>[2x]MLLEAIFHEAK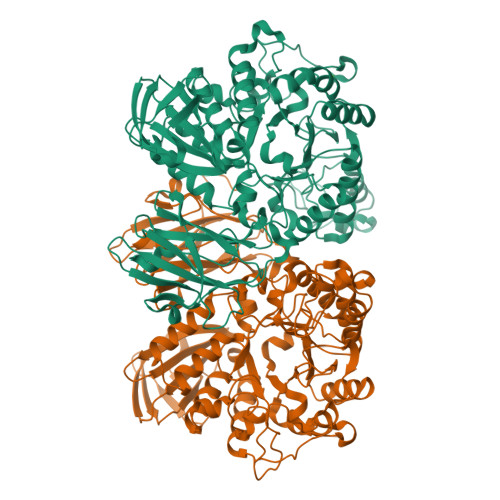GSYAYPISETQLRVRLRAKKGDVVRCEVLYADRYASPEEELAHALAGKAGSDERFDYFEALLECSTKRVKYVFLLTGPQGEAVYFGETGFSAERSKAGVFQYAYIHRSEVFTTPEWAKEAVIYQIFPERFANGDPSNDPPGTEQWAKDARPRHDSFYGGDLKGVIDRLPYLEELGVTALYFTPIFASPSHHKYDTADYLAIDPQFGDLPTFRRLVDEAHRRGIKIILDAVFNHAGDQFFAFRDVLQKGEQSRYKDWFFIEDFPVSKTSRTNYETFAVQVPAMPKLRTENPEVKEYLFDVARFWMEQGIDGWRLDVANEVDHAFWREFRRLVKSLNPDALIVGEIWHDASGWLMGDQFDSVMNYLFRESVIRFFATGEIHAERFDAELTRARMLYPEQAAQGLWNLLDSHDTERFLTSCGGNEAKFRLAVLFQMTYLGTPLIYYGDEIGMAGATNPDCRRPMIWEEKEQNRGLFEFYKELIRLRHRLASLTRGNVRSWHADKQANLYAFVRTVQDQHVGVVLNNRGEKQTVLLQVPESGGKTWLDCLTGEEVHGKQGQLKLTLRPYQGMILWNGR> AQYYPGTTKVAQNRRNFCNPEYELEKLREISDEDVVKILGHRAPGEEYPSVHPPLEEMDEPEDAIREMVEPIDGAKAGDRVRYIQFTDSMYFAPAQPYVRSRAYLCRYRGADAGTLSGRQIIETRERDLEKISKELLETEFFDPARSGVRGKSVHG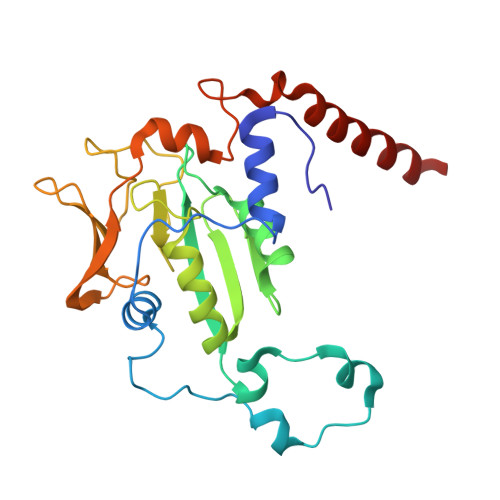HSLRLDEDGMMFDMLRRQIYNKDTGRVEMVKNQIGDELDEPVDLGEPLDEETLMEKTTIYRVDGEAYRDDVEAVEIMQRIHVLRSQGGFN> GSLKGTQSLNPHNDYCQHFVDTGHRPQNFIRDVGLADRFEEYPKLRELIRLKDELIAKSNTPPMYLQADIEAFDIRELTPKFDVILLEPPLEEYYRETGITANEKCWTWDDIMKLEIDEIAAPRSFIFLWCGSGEGLDLGRVCLRKWGYRRCEDICWIKTNKNNPGKTKTLDPKAVFQRTKEHCLMGIKGTVKRSTDGDFIHANVDIDLIITEEPEIGNI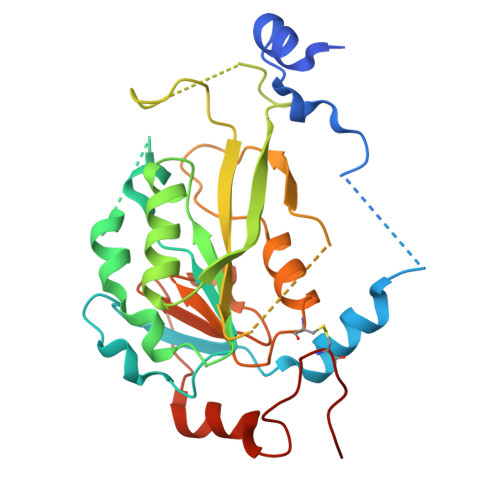EKPVEIFHIIEHFCLGRRRLHLFGRDSTIRPGWLTVGPTLTNSNYNAETYASYFSAPNSYLTGCTEEIERL>[2x]GSHMLFDFENDQVPSNIHFLNARASIETYTGINGEPSKGLKLAMQSKQHSYTGLAIVPEQPWDWSEFTSASLYFDIVSVGDHSTQFYLDVTDQNGAVFTRSIDIPVGKMQSYYAKLSGHDLEVPDSGDVNDLNLASGLRSNPPTWTSDDRQFVWMWGVKNLDLSGIAKISLSVQSAMHDKTVIIDNIRIQPNPPQDENFLVGLVDEFGQNAKVDYKGKIHSLEELHAARDVELAELDGKPMPSRSKFGGWLAGPKLKATGYFRTEKINGKWMLVDPEGYPYFATGLDIIRLSNSSTMTGYDYDQATVAQRSADDVTPEDSKGLMAVSEKSFATRHLASPTRAAMFNWLPDYDHPLANHYNYRRSAHSGPLKRG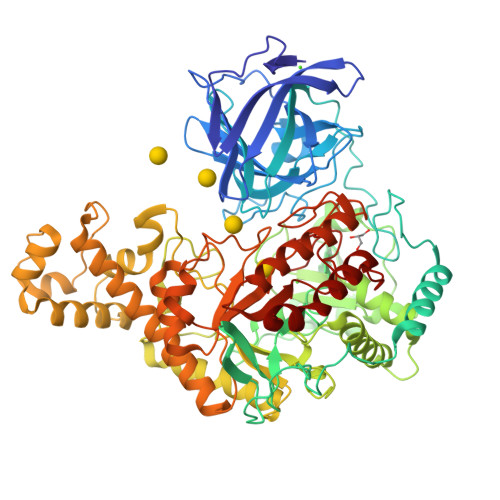EAYSFYSANLERKYGETYPGSYLDKWREVTVDRMLNWGFTSLGNWTDPAYYDNNRIPFFANGWVIGDFKTVSSGADFWGAMPDVFDPEFKVRAMETARVVSEEIKNSPWCVGVFIDNQKSFGRPDSDKAQYGIPIHTLGRPSEGVPTRQAFSKLLKAKYKTIAALNNAWGLKLSSWAEFDLGVDVKALPVTDTLRADYSMLLSAYADQYFKVVHGAVEHYMPNHLYLGARFPDWGMPMEVVKAAAKYADVVSYNSYKEGLPKQKWAFLAELDKPSIIGEFHIGAMDHGSYHPGLIHAASQADRGEMYKDYMQSVIDNPYFVGAHWFQYMDSPLTGRAYDGENYNVGFVDVTDTPYQEMVDAAKEVNAKIYTERLGSK>[8x]MATRQRESSITSCCSTSSMDENDEGVRGTCEDASLCKRFAVSIGYWHDPYIQHFVRLSKERKAPEINRGYFARVHGVSQLIKAFLRKTECHCQIVNLGAGMDTTFWRLKDEDLLSSKYFEVDFPMIVTRKLHSIKCKPPLSSPILELHSEDTLQMDGHILDSKRYAVIGADLRDLSELEEKLKKCNMNTQLPTLLIAECVLVYMTPEQSANLLKWAANSFER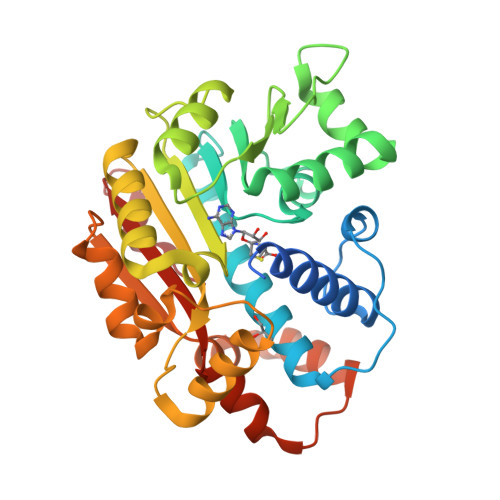AMFINYEQVNMGDRFGQIMIENLRRRQCDLAGVETCKSLESQKERLLSNGWETASAVDMMELYNRLPRAEVSRIESLEFLDEMELLEQLMRHYCLCWATKGGNELGLKEITY>SNAMIRKYRYGAPFDTEALTEKIETAEEAFPYGEISQKEGFAFTYIMDEDDIVYGLGESNRGINKRGYCYISNCTDDPIHTEDKRSLYGAHNFIIVSGKTTFGLFFDYPSKLTFDIGYTRMDTLKVSCENADLDIYVIEGENAYDIVKQFRRVIGRSYIPPKFAFGFGQSRWGYTTKEDFRAVAKGYRENHIPIDMIYMDIDYMQDFKDFTVNEKNFPDFPEFVKEMKDQELRLIPIIDAGVKVEKGYEVYEEGVKNNYFCKREDGSDFVAAVWPGDTHFPDMLNPEARKWFGDKYRFLIDQGIEGFWNAMNEPAIFYSSEGLAEAKEFAGEFAKDTEGKIHPWAMQAKMKDIVNSPEDYKRFYHNVNGKKIRHDKVHNLFGYNMTRAAGEAFERIDPEKRFLMFSRSSYIGMHRYGGIWMGDNKSWWSHILLNLKMLPSLNMCGFMYTGADLGGFGDDTTRDLLLRFLALGVFTPLMRDHAAEGTREQECYQFENIEDFRSVINARYRLVPYLYSEYMKAALNDDMYFKPLGFVYPDDKMAIRVEDQLMLGNE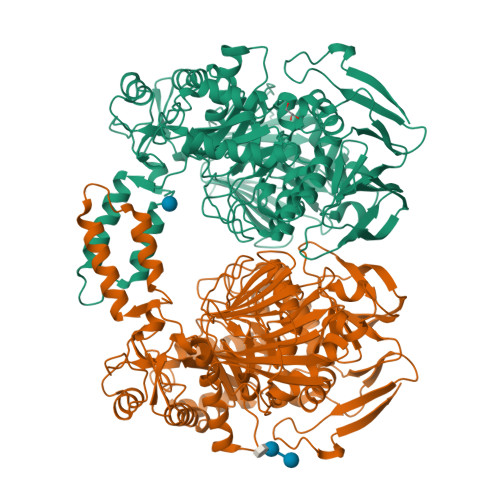IMIAPVYEQNARGRYVYLPEEMKFIKFMPDGSISEEVLEKGVHYVDVALNEVPLFIRSGKCIPVAEAAECVKDIDTENMQLIGYEGSSYTLYEDDGIHKDYDKKENYRVLTK[2x]>DISTVPDETYDALKLDRGKATPKETYEALVKRYKDPAHGAGKGTMGDYWEPIAISIYMDPNTFYKPPVSPKEVAERKDCVECHSDETPVWVRAWKRSTHANLDKIRNLKSDDPLYYKKGKLEEVENNLRSMGKLGEKETLKEVGCIDCHVDVNKKDKADHTKDIRMPTADTCGTCHLREFAERESERDTMVWPNGQWPAGRPSHALDYTANIETTVWAAMPQREVAEGCTMCHTNQNKCDNCHTRHEFSAAESRKPEACATCHSGVDHNNWEAYTMSKHGKLAEMNRDKWNWEVRLKDAFSKGGQNAPTCAACHMEYEGEYTHNITRKTRWANYPFVPGIAENITSDWSEARLDSWVLTCTQCHSERFARSYLDLMDKGTLEGLAKYQEANAIVHKMYEDGTLTGQKTNRPNPPEPEKPGFGIFTQLFWSKGNNPASLELKVLEMAENNLAKMHVGLAHVNPGGWTYTEGWGPMNRAYVEIQDEYTKMQELSALQARVNKLEGKQTSLLDLKGTGEKISLGGLGGGMLLAGALALIGWRKRKQTRA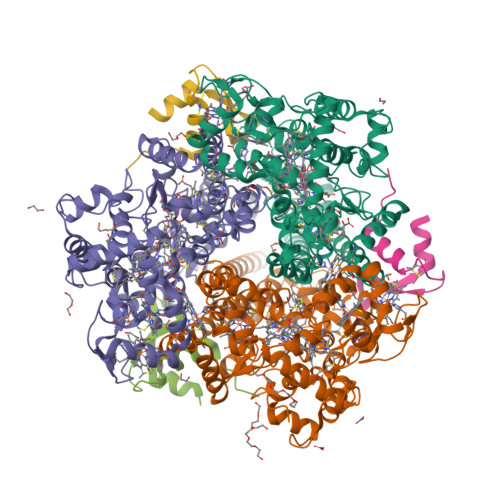[3x];>SGNLESSLAPISAKDMLDYLACKDKKPTDVVKSHTEVENGKIVRVKCGDIVALVQKAREQSGDAWQGGY[3x]>GMADPSLHHEAQPLKFIAVDYCPESCTHSPESSTITLTFDHRGGSRWRSTTRFQYGTFSSLIQCPKGNTSGLNFNIYLSSLEGDKSQDAIDFEFLGKDKRIVQTNYYTAGTGNREAIHDLGFDCSDGFHEYVIKWGPDLIQWLIDGKVIRSVRADGEGFPQKPMFLY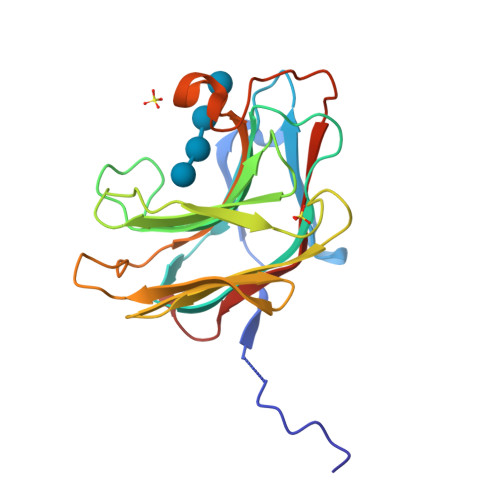ASVWDASYIDEGRWTGPYVGCDAPYICLYKNVNVPVGTAVE[2x]> SLENENQLTHQFPTLSRWNPMFISDVHKISFHPHLQRYIGFWMGFPIRWIQIVGYIAAIDIYEGKHVLTVDDCSGMVLRVVFIIQDDFSMSKRAISMSPGNVVCVFGKINSFRSEVELIAQSFEELRDPNDEWKAWQKRMRYKKNLTKISKNHHSIIRT;> PLGSDSAKLIFINQINDCKDGQKLRFLG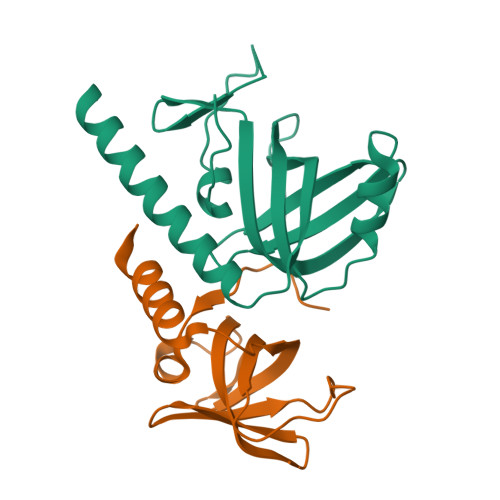CVQSYKNGILRLIDGSSSVTCDVTVVLPDVSIQKHEWLNIVGRKRQDGIVDVLLIRSAVGINLPRYRQMVSERQKCD>[2x]MRGSHHHHHHGLVPRGSMIRTMLQGKLHRVKVTHADLHYEGSACAID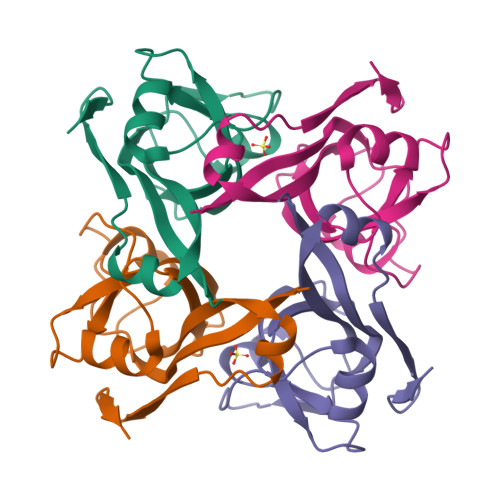QDFLDAAGILENEAIDIWNVTNGKRFSTYAIAAERGSRIISVNGAAAHCASVGDIVIIASFVTMPDEEARTWRPNVAYFEGDNEMKRTAKAIPVQVA>MNKPSFLLVGLLVVSGVLGAAETKVKYPDGFRSWYHVKSMVIQPGHPLENPFGGIHHVYANAEAIQGLRGGNYPDGAVLVFDLFDYQEDNHALVEGKRKLIGVMERDAKRFSATGGWGYEGFGEGKPDKRLVTDGGQGCFGCHAAQKESQYVFSRLRD[2x]

A widely applicable approach is the use of photocaged substrates, where the photocage is soaked into the crystal in advance and then activated using a laser pulse to provide uniform initiation of the reaction throughout the crystal. This work characterizes photocage release of nitric oxide and binding of this ligand to two heme protein systems, cytochrome c′-β and dye-decolourizing peroxidase B using a fixed target sample delivery system. In this work, we describe a thorough characterization of the application of the NO photocage N,N′-bis-(carb­oxy­methyl)-N,N′-di­nitroso-1,4-phenyl­enedi­amine (henceforth referred to as NO cage) to room-temperature microcrystals of two proteins: a gas binding cytochrome c′ (McCP-β) and a dye-decolourizing peroxidase B (DtpB). Laser parameters for photoactivation are systematically explored, and time-resolved structures over timescales ranging from 100 µs to 1.4 s using synchrotron and XFEL beamlines are described. We have demonstrated a sample and time efficient approach using fixed targets to carry out time-resolved SSX and SFX experiments with an NO photocage over the microsecond to second time regimes.

An initial high power laser experiment delivering 1600 µJ (580 nJ µm−2) of laser energy to the sample over 10 ms of 50 kHz PORTO laser pulses showed NO binding with an occupancy of 1.0 (1.80 Å resolution) but with notably different 2Fo − Fc and omit density features to those from subsequent data collections. This high laser power requirement was due, at least in part, to an initial sub-optimal experimental setup where the fixed targets were orientated with the narrow end of the funnel-like apertures facing the laser beam, and with Mylar sealing both sides. In this orientation, the chip acts as an aperture, blocking a significant fraction of laser light resulting in inefficient excitation and causing only part of the crystal volume seen by X-rays to be illuminated by the laser. The unexpected electron density features may therefore be due to laser induced damage (though a loss in diffracting power was not observed) or non-uniform excitation.PICRIC 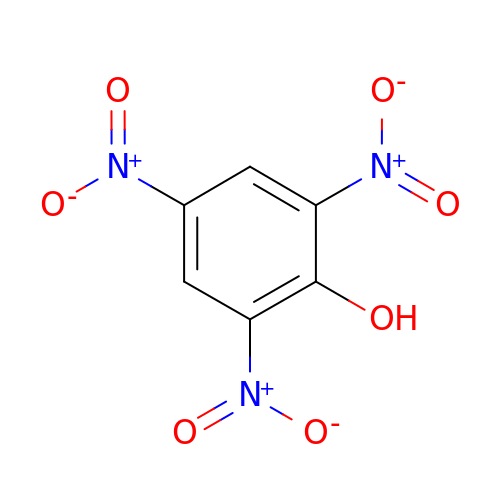ACID | C6 H3 N3 O7 | OXNIZHLAWKMVMX-UHFFFAOYSA-N> MSRNDKEPFFVKFLKSSDNSKCFFKALESIKEFQSEEYLQIITEEEALKIK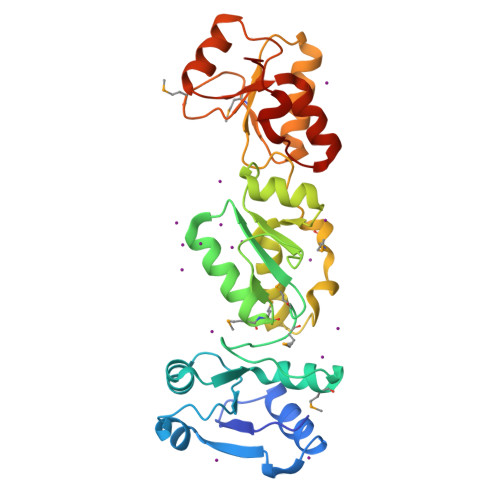ENDRSLYICDPFSGVVFDHLKKLGCRIVGPQVVIFCMHHQRCVPRAEHPVYNMVMSDVTISCTSLEKEKREEVHKYVQMMGGRVYRDLNVSVTHLIAGEVGSKKYLVAANLKKPILLPSWIKTLWEKSQEKKITRYTDINMEDFKCPIFLGCIICVTGLCGLDRKEVQQLTVKHGGQYMGQLKMNECTHLIVQEPKGQKYECAKRWNVHCVTTQWFFDSIEKGFCQDESIYKTEPR> MSYQYVNVVTINKVAVIEFNYGRKLNALSKVFIDDLMQALSDLNRPEIRCIILRAPSGSKVFSAGHDIHELPSGGRDPLSYDDPLRQITRMIQKFPKPIISMVEGSVWGGAFEMIMSSDLIIAASTSTFSMTPVNLGVPYNLVGIHNLTRDAGFHIVKELIFTASPITAQRALAVGILNHVVEVEELEDFTLQMAHHISE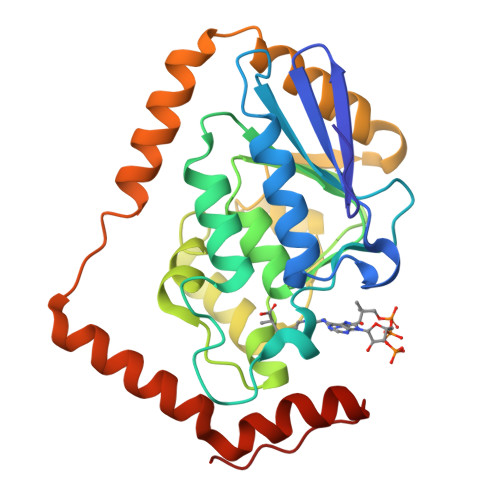KAPLAIAVIKEELRVLGEAHTMNSDEFERIQGMRRAVYDSEDYQEGMNAFLEKRKPNFVGH>MKKIALIIGSMIAGGIISAAGFTWVAKAEPPAEKTSTAERKILFWYDPMYPNTRFDKPGKSPFMDMDLVPKYADEESSASGVRIDPTQTQNLGVKTATVTRGPLTFAQSFPANVSYNEYQYAIVQARAAGFIDKVYPLTVGDKVQKGTPLLDLTIPDWVEAQSEYLLLRETGGTATQTEGILERLRLAGMPEADIRRLIATQKIQTRFTLKAPIDGVITAFDLRAGMNIAKDNVVAKIQGMDPVWVTAAIPESIAWLVKDASQFTLTVPARPDKTLTIRKWTLLPGVDAATRTLQLRLEVDNADEALKPGMNAWLQLNTASEPMLLIPS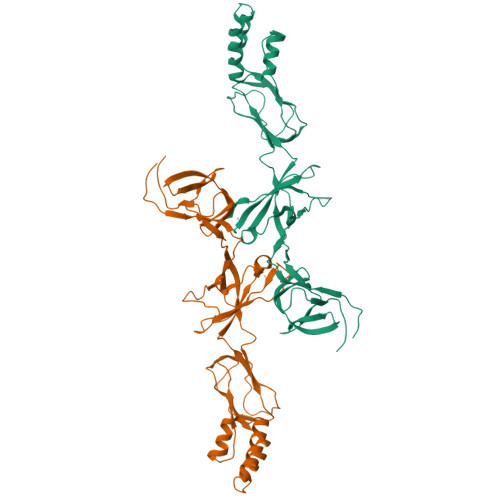QALIDTGSEQRVITVDADGRFVPKRVAVFQASQGVTALRSGLAEGEKVVSSGLFLIDSEANISGALERMRSESATHAHHHHHHH[2x]>[2x]MRTLYPEITPYQQGSLKVDDRHTLYFEQCGNPHGKPVVMLHGGPGGGCNDKMRRFHDPAKYRIVLFDQRGSGRSTPHADL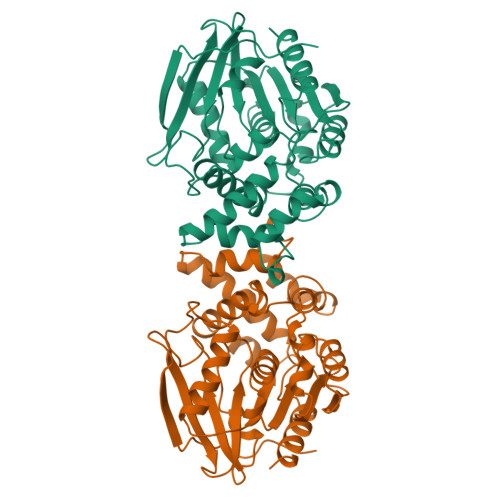VDNTTWDLVADIERLRTHLGVDRWQVFGGSWGSTLALAYAQTHPQQVTELVLRGIFLLRRFELEWFYQEGASRLFPDAWEHYLNAIPPVERADLMSAFHRRLTSDDEATRLAAAKAWSVWEGATSFLHVDEDFVTGHEDAHFALAFARIENHYFVNGGFFEVEDQLLRDAHRIADIPGVIVHGRYDVVCPLQSAWDLHKAWPKAQLQISPASGHSAFEPENVDALVRATDGFA IRE1 integrates multiple functional domains into a single ER-membrane-spanning protein. The lumenal domain senses unfolded proteins in the ER through indirect and direct mechanisms: as a result, it undergoes dimerization and subsequent oligomerization. The association of the lumenal domain promotes dimerization and oligomerization of the cytoplasmic kinase-RNase tandem domain. The cytoplasmic domain has been shown to self-associate via different surface contacts, where a back-to-back (B2B) configuration is believed to fulfill the essential structural requirements for RNase activation.

The B2B dimeric and oligomeric IRE1 complexes are stabilized by phosphorylation of the kinase activation loop, which in human IRE1 occurs on residues S724, S726, S729, making phosphorylated IRE1 (IRE1-3P) the most active form of the RNase enzyme. We determined the crystal structures of G-9807 and G-1749 in complex with IRE1-0P at about 2 Å resolution. The structures are shown in Fig. 2 together with the structures of AMG-18-bound-31 and apo IRE1, including the first reported crystal structure of human apo IRE1-3P. All structures show IRE1 as a B2B dimer, with extensive overlay of the RNase domains, but some differences in the kinase domains, especially in the conformation of the activation loop and αEF-αF loop. A possible reason for this is the stabilization of the extended activation loop conformation by the extensive hydrogen bonding network that the phosphates on S724, S726, and S729 form with the backbone and sidechains on the activation loop. The resulting rigidification would make the opening of the front pocket, which would require an upward shift of the activation loop, energetically unfavorable, depending perhaps on the number of phosphates present on the loop. A similar stabilization effect was observed in the IRE1-3P sample. This suggests that stabilization of the activation loop in an extended conformation by phosphorylation or binding to allosteric RNase activators may stabilize IRE1 B2B dimers through widespread rigidification of the kinase in the monomer context. In one case, phosphorylations on the kinase activation loop can stabilize an extended conformation of the loop, rigidifying the kinase and stabilizing the B2B dimer as a consequence.

>GSSPSLEQDDGDEETSVVIVGKISFCPKDVLGHGAEGTIVYRGMFDNRDVAVKRILPECFSFADREVQLLRESDEHPNVIRYFCTEKDRQFQYIAIELCAATLQEYVEQKDFAHLGLEPITLLQQTTSGLAHLHSLNIVHRDLKPHNILISMPNAHGKIKAMISDFGLCKKLAVGRHSFSRRSGVPGTEGWIAPEMLSEDCKENPTYTVDIFSAGCVFYYVISEGSHPFGKSLQRQANILLGACSLDCLHPEKHEDVIARELIEKMIAMDPQKRPSAKHVLKHPFFWSLEKQLQFFQDVSDRIEKESLDGPIVKQLERGGRAVVKMDWRENITVPLQTDLRKFRTYKGGSVRDLLRAMRNKKHHYRELPAEVRETLGSLPDDFVCYFTSRFPHLLAHTYRAMELCSHERLFQPYYFHEPPEPQPPVTPDALGNS[4x]> DGVSILQTASSGLTSLTNSLQRIRQLAVQASNGPLSASDASALQQEVAQQISEVNRIASQTNYNGKNILDGSAGTLSFQVGANVGQTVSVDLTQSMSAAKIGGGMVQTGQTLGTIKVAIDSSGAAWSSGSTGQETTQINVVSDGKGGFTFTDQNNQALSSTAVTAVFGSSTAGTGTAASPSFQTLALSTSATSALSATDQANATAMVAQINAVNKPQTVSNLDISTQTGAYQAMVSIDNALATVNNLQATLGAAQNRF

To date, one of the main candidate antigens is bacterial flagellin (FliC), which assembles to form the flagellar filament that supports bacterial motility. Interestingly, FliC is recognized as a pathogen associated molecular pattern (PAMP) by Toll-like receptor 5 (TLR5) and by nucleotide-binding oligomerization domain (NOD)-like receptor C4 (NLRC4), activating both innate and adaptive immunity. Flagellins vary in dimension (28–65 kDa) and contain at least two essential highly conserved domains, D0 and D1 that mediate assembly of the flagellar filament, and may contain a second (D2) or third (D3) variable domain. FliCBp constitutes a major target for vaccine discovery initiatives to elicit protective immunity against B. pseudomallei infections.

We also report the 1.3Å resolution FliCBp crystal structure as the basis for in silico epitope predictions using two diverse computational methods. FliCBp (residues 25 to 378) was crystallized using the sitting drop vapor diffusion method, as described in the Materials and Methods section. Electron density was visible for residues 69–326; the first 44 N-terminal residues and the 52 C-terminal residues were absent, however experimental epitope mapping revealed two immunocaptured peptides containing N-terminal residue 37 and residue 361, therefore the residues that are not visible in the electron density are likely to be present in disordered regions of the protein. Typically, removal of the D0 domain is necessary for successful crystallization. This was not the case for FliCBp where, however, the first 44 N-terminal residues (corresponding to the D0 domain) are not visible in the electron density map because of structural disorder. Overall, FliCBp adopts the canonical flagellin fold and presents two domains, a conserved D1 domain (residues 69–167, 287–326), and a variable D2 domain (168 and 286). D1 forms a helical rod (α1, α2 and α5) involving residues contributed by both the N-terminus (residues 69–170) and C-terminus (residues 285–326), a β-hairpin domain (β1-β2) and a 310 α-helix (η1). Domain D2 (residues 172–287) contains a three-stranded antiparallel β-sheet, two α−helices (α3 and α4) and two 310 α-helices (η2 and η3). Domain D2 is connected to D1 via two anti-parallel regions that house two short 310 α-helices (η1 and η3) that interact with each other, thus stabilizing the relative positions of the two domains. F96-111 is housed in domain D1 and is composed of two short α-helical segments at the C- and N- termini of α-helices 1 and 2, connected by a short loop. The third predicted peptide F270-288, is located in domain D2 and is formed by α-helix 4, the 310 α-helices η3, and their connecting loop region.> KPKGHPHMNSIRIDGDITLGGLFPVHGRGSEGKPCGELKKEKGIHRLEAMLFALDRINNDPDLLPNITLGARILDTCSRDTHALEQSLTFVQALIEKDGTEVRCGSGGPPIITKPERVVGVIGASGSSVSIMVANILRLFKIPQISYASTAPDLSDNSRYDFFSRVVPSDTYQAQAMVDIVRALKWNYVSTVASEGSYGESGVEAFIQKSREDGGVCIAQSVKIPREPKAGEFDKIIRRLLETSNARAVIIFANEDDIRRVLEAARRANQTGHFFWMGSDSWGSKIAPVLHLEEVAEGAVTILPKRMSVRGFDRYFSSRTLDNNRRNIWFAEFWEDNFHCKLSRHALKKGSHVKKCTNRERIGQDSAYEQEGKVQFVIDAVYAMGHALHAMHRDLCPGRVGLCPRMDPVDGTQLLKYIRNVNFSGIAGNPVTFNENGDAPGRYDIYQYQLRNDSAEYKVIGSWTDHLHLRIERMHWPGSGQQLPRSICSLPCQPGERKKTVKGMPCCWHCEPCTGYQYQVDRYTCKTCPYDMRPTENRTGCRPIPIIKLEWGSPWAVLPLFLAVVGIAATLFVVITFVRYNDTPIVKASGRELSYVLLAGIFLCYATTFLMIAEPDLGTCSLRRIFLGLGMSISYAALLTKTNRIYRIFEQGKRSVSAPRFISPASQLAITFSLISLQLLGICVWFVVDPSHSVVDFQDQRTLDPRFARGVLKCDISDLSLICLLGYSMLLMVTCTVYAIKTRGVPETFNEAKPIGFTMYTTCIVWLAFIPIFFG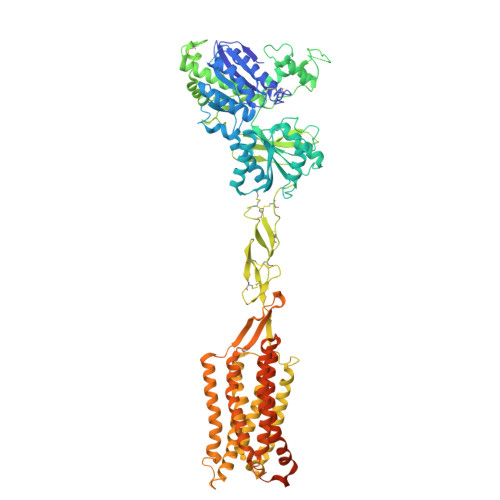TSQSADKLYIQTTTLTVSVSLSASVSLGMLYMPKVYIILFHPEQNVPKRKRSLKAVVTAATMSNKFTQKGNFRPNGEAKSELCENLEAPALATKQTYVTYTNHAI> MIYMLDTNIIIYLMKNRPKIIAERVSQLLPNDRLVMSFITY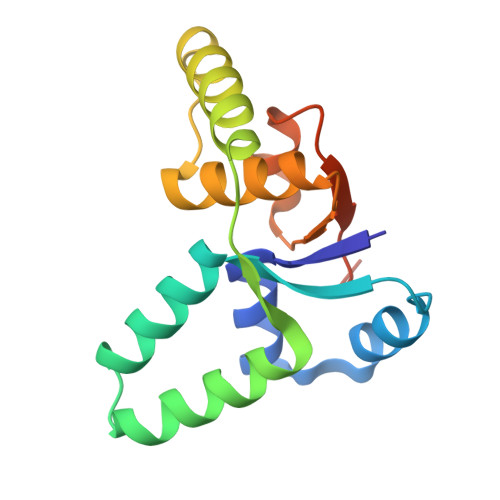AELIKGAFGSQNYEQSIRAIELLTERVNVLYPNEQICLHYGKWANTLKKQGRPIGNNDLWIACHALSLNAVLITHNVKEFQRITDLQWQDWTKLLEHHHHHH>GHMKASSRRTISQNKRRYRKDGFDLDLTYVTDHV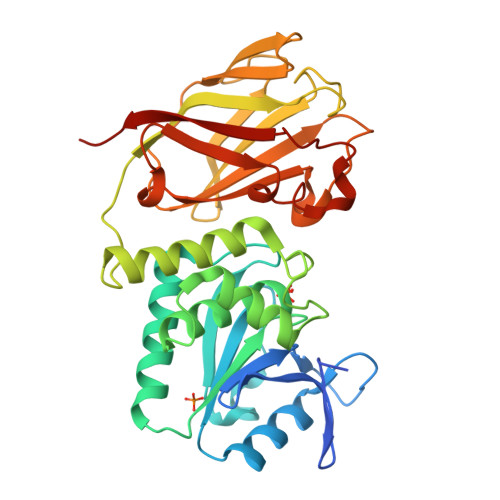IAMSFPSSGRQSLFRNPIGEVSRFFKTKHPDKFRIYNLCSERGYDETKFDNHVYRVMIDDHNVPTLVDLLKFIDDAKVWMTSDPDHVIAIHSKGGKGRTGTLVSSWLLEDGKFDTAKEALEYFGSRRTDFEVGDVFQGVETASQIRYVGYFEKIKKNYGGQLPPMKKLKVTGVTITAIQGVGRGNGSDLSMQIVSERQEVLLCKFAEGYNCALQYDATDDCVTCEVKNCPVLAGDIKVRFMSTSKSLPRGYDNCPFYFWFNTSLVEGDHVTLKREEIDNPHKKKTWKIYRDNFTVKLTFSDAEDI[2x]> XCAIDQDFLDAAGILENEAIDIWNVTNGKRFSTYAIAAERGSRIISVNGAAAHCASVGDIVIIA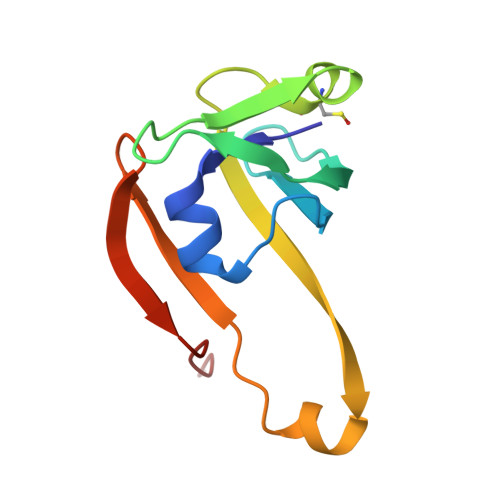SFVTMPDEEARTWRPNVAYFEGDNEMKRTAKAIPVQVA>[3x]MPFVDLEVPTMTTPTPAATPARPRVLTGDRPTGALHLGHLAGSLQ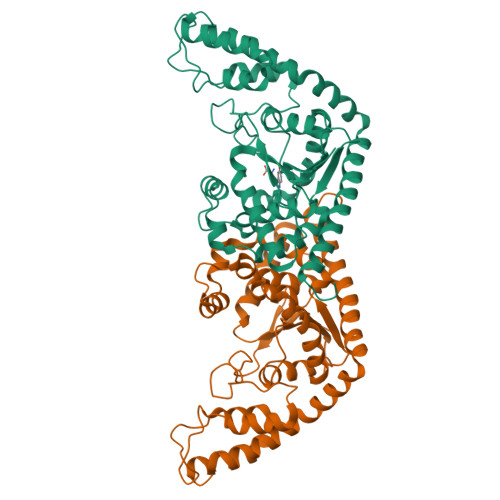NRVRLQDEAELFVLLADVQALTDHFDRPEQVRENVLAVALDYLAAGLDPQKTTCVVQSAVPELAELTVYFLNLVTVSHLRQNPTVKAEIAQKGYGERVPAGFFVYPVSQAADIAAFGATLVPVGDDQLPMLEQTREIVRRFNALYAPVLAEPQAQLSRVPRLPGLDGQAKMSKSLGNAIALGDSADEVARKVMGMYTDPGHLRASDPGRVEGNPVFTFLDAFDPDPARVQALKDQYRAGGLGDVKVKKHLIDVLNGVLAPIRTRRAEYERDPDAVLRFVTEGTARGREVAAQTLGQVRRAMRLFGH> RAEKTGLTLALILLLTFFSLIVYAAKGLKIDIPTCVTDVEPFQEGKLIKHGDKRYELHILARMWYFDFNKGATEIKIPVGSVVDI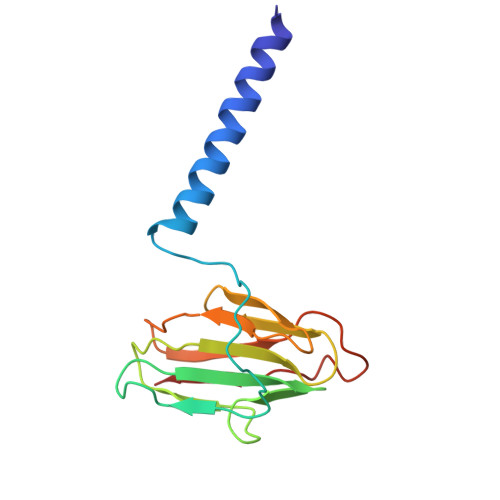FTTSKDVVHGVHIHGTNYNVMAIPGTVGYMRIKFEKPGVYHVVCHEFCGVGHHAMQGKIIVE> MQELYLLGVVPSRRFEAVVNSLSKTLDGPKTILEFWVVYRPKDVPPNLPRQPDSWLRLCSNIESHDETDT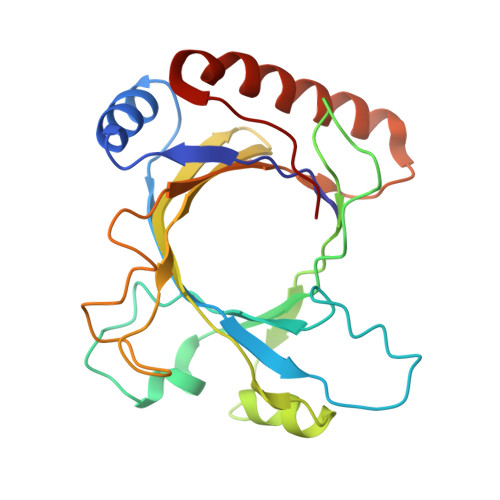EWSKNTQWSMYLEGNSEPKREDKCGIRPVNRAKLTNGSVTEFVEKMGYEFSHEYIIQGLEYFFFDTTVRIYQTLIPSQQRSIKPPFHPMNEEQPWILHVYTHVADASNQVAMAKAEANLTKVKTLLSAFCDLKNVRL>[2x]MRSRRVDVMDVMNRLILAMDLMNRD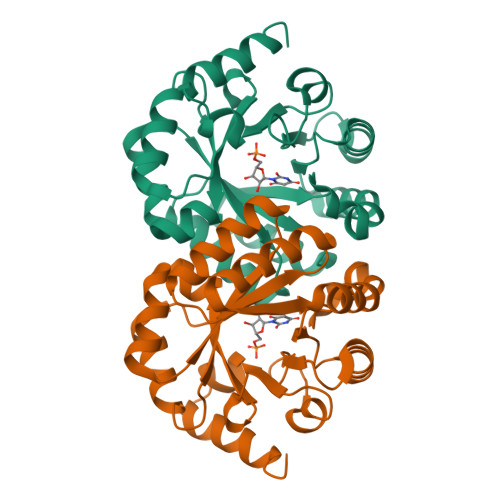DALRVTGEVREYIDTVKIGYPLVLSEGMDIIAEFRKRFGCRIIADFKVADIPETNEKICRATFKAGADAIIVHGFPGADSVRACLNVAEEMGREVFLLTEMSHPGAEMFIQGAADEIARMGVDLGVKNYVGPSTRPERLSRLREIIGQDSFLISPGVGAQGGDPGETLRFADAIIAGRSIYLADNPAAAAAGIIESIKDLLNP>[12x]MTIEYATRHRARSFIPPEPGKPYFIEKGLGDRAHLFGDLITIYAGGEQTENTFNFFTCEGPKGEVIPAHSHADTYEVFYITQGAVRLFVEDLEGEQHEKLLTPGDFG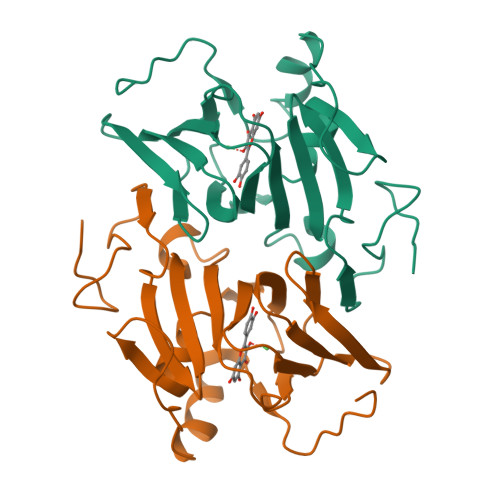FVPKNCVHAYRMERHHSQVVGVAAGPGGTFERFFESLGTPAEELGLPVRPFVPEPEKFRTVPEQYDVRFRPDHQWHTGS> MKLKSILSAAIFTGLFSTAGIAGTITSQDDNVVVGYWHNWCDGRGYQGGNAPCVELKTVNPQYNVVNISFMKVY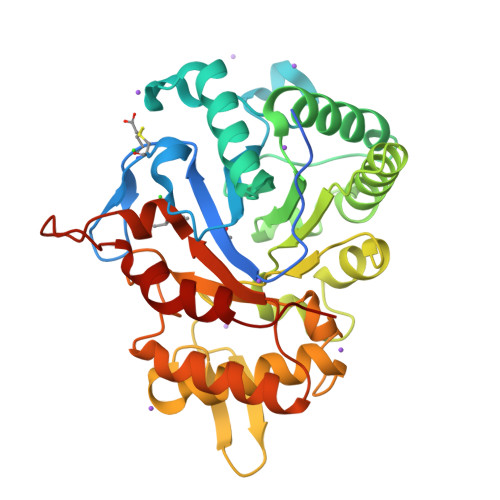DIAEGRIPTFKLDPTIALSEAEFIAQIDTLNSQGRSVLIALGGADAHIELTRGDEDALAAEIIRLTDLYGFDGLDIDLEQAAITAKDNQFVIPAALKMVKEHYRKTGDNFMITMAPEFPYLTANGAYTPYLTELDGYYDFINPQFYNQGGDGLWIEGVGWIAQNNDALKEEFIYYIADSLINGTRNYHKIPHDKLVFGLPSNIDAAATGYIQDPQDLYKAFDRLKAQGQPLRGVMTWSVNWDMGTDAANNSYNQQFIKDYGNFIHNQLPPV5-fluoro-N-[5-(4-methylpiperazin-1-yl)pyridin-2-yl]-4-[(4R)-4-methyl-5,6,7,8-tetrahydro-4H-pyrazolo[1,5-a]azepin-3-yl]pyrimidin-2-amine 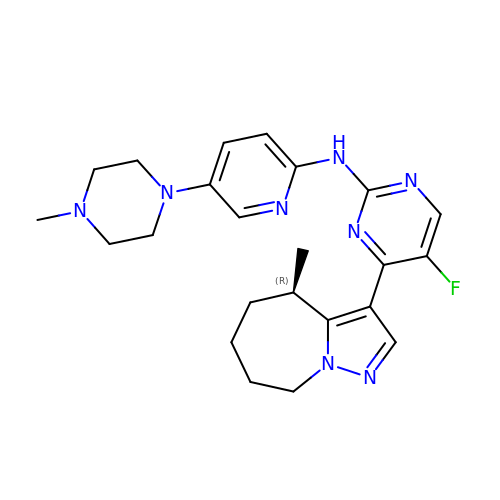| C23 H29 F N8 | UHCMUGYUWQCODZ-MRXNPFEDSA-N> SNADDYTAGKEYVELS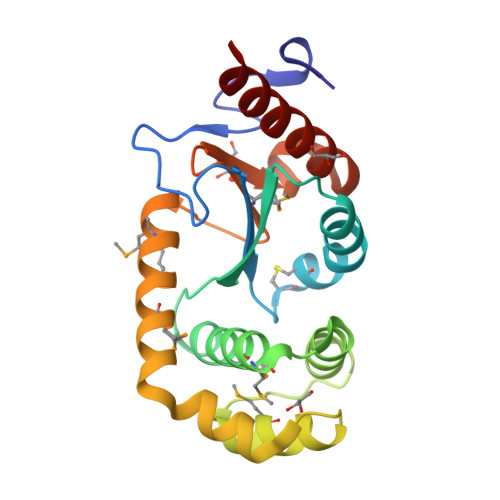SPVPVSQPGKIEVVELFWYGCPHCYAFEPTIVPWSEKLPADVHFVRLPALFGGIWNVHGQMFLTLESMGVEHDVHNAVFEAIHKEHKKLATPEEMADFLAGKGVDKEKFLSTYNSFAIKGQMEKAKKLAMAYQVTGVPTMVVNGKYRFDIGSAGGPEETLKLADYLIEKERAAAKK1-[1-[[4-(3-chloranylphenoxy)quinolin-2-yl]methyl]piperidin-4-yl]-5-methyl-pyrimidine-2,4-dione 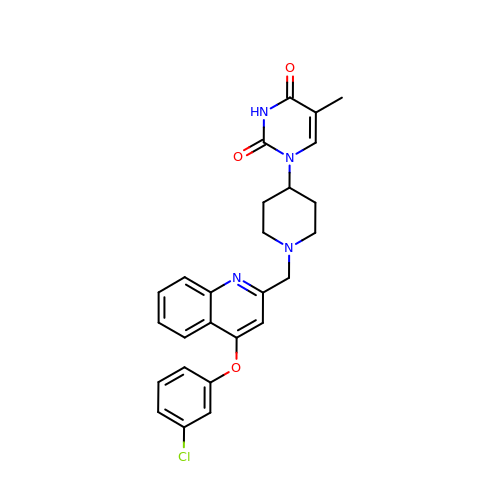| C26 H25 Cl N4 O3 | DAZGAHYHWTYXTL-UHFFFAOYSA-N One protein family common to humans, C. parvum and in fact all eukaryotes is the group of tyrosine 3-monooxygenase/tryptophan 5-monooxygenase activation proteins (YWHA), also known as 14-3-3 proteins. All 14-3-3 proteins are dimers, with each subunit comprised of nine α-helices framing a peptide-binding cleft. The dimer is shaped like the letter “W” from one angle, with an un-partitioned bicameral pocket where a substrate protein is held at two typically phosphorylated sites in the two component clefts. The parasite Cryptosporidium parvum has three 14-3-3 proteins: Cp14ε, Cp14a and Cp14b, with only Cp14ε similar to human 14-3-3 proteins in sequence, peptide-binding properties and structure.

Structurally, Cp14a features the classical 14-3-3 dimer but with a uniquely wide pocket and a disoriented RRY triad potentially incapable of binding phosphopeptides. Cp14a shares limited sequence identity with Cp14ε and all other known proteins. First, while the Cp14a structure also adopts the classic dimeric α-helical structure, it stands out by virtue of its unusual width. More strikingly, Cp14a is further distinguished by the natural absence of a C-terminal tail ensuing the last helix. Even the second arginine and the ensuing tyrosine are skewed in their orientations with respect to what is typical in other 14-3-3 proteins, with or without ligands bound. This is the first known instance of a disoriented 14-3-3 triad (superposed on Cp14ε for comparison in Fig. 4D). The mode of dimerization of Cp14a deviates from that of other 14-3-3 proteins. While the two subunits form an aperture similar to that in the human 14-3-3 proteins and Cp14ε, the side chain interactions around the aperture are primarily hydrophobic, with Cys26 and Met70 of opposite chains occupying the position of the Arg-Glu salt bridge conserved in most other homologs. One intuitive conclusion is that this protein supports a large substrate; however, its disoriented Arg-Arg-Tyr triad, the lack of a C-terminal tail and our negative screening results make this C. parvum chaperone even more divergent from others and introduces the possibility that this is a degenerate 14-3-3 protein, or at least one that is functionally unique.

> GEMDERLLQKYRAQVFEWGGCFDKMFEALKSLIYLSEFENSEFDDEERHLLTLCIKHKISDYRTMTSQVLQEQTKQLNNDELVKICSEYVFSLRKDIKAFLQSFEDCVDRLVEKSFFSKFFKLKVKSDISRYKLEFGLCSLEDSKKIHQDAFTLLCEHPDKIEQLPLGFIQNLAYILSEKYGEKKQVFNMLNSLGKILELQIKEQENMDRKAQITVYLQGIKDYIEK> GMTAPADTSTLESRVGHYYQMEDTYLVGREKVREFARAVQDYHPA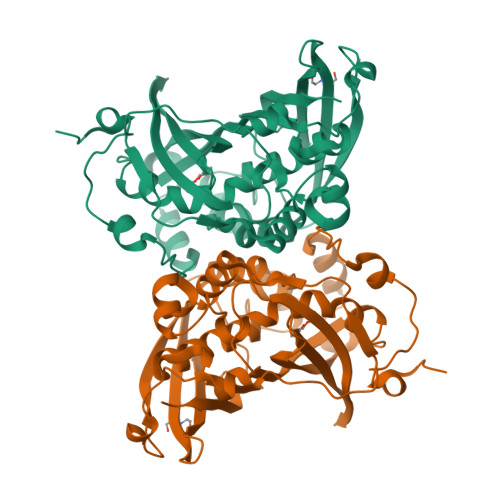HWNLATAADLGHPGLIAPLTFTSAPAMACNQRMFESVVVGYDMYLQTEEVFEQHRPIVEGDELSIDIELTSVRRIAGRDLITVTNTFTDTAGEVVHTLHTTVVGITAEDVDPAIRPAVQGVMMHGINMLGVEETNAPYEKTVRPEGELRIAQGGATRTPTSLNFDDLKVGEELPVHTARLSRGDLVNYAGVAGDANPLHWDENIAKLAGQPDVIAHGMLTMGLGAGFVSSWSGDPGAITRYAVRLSQPAVVPAEGTEIEYSGRIKSLDPETRTGVVIVAAKSGGRKIFGLATATIRFS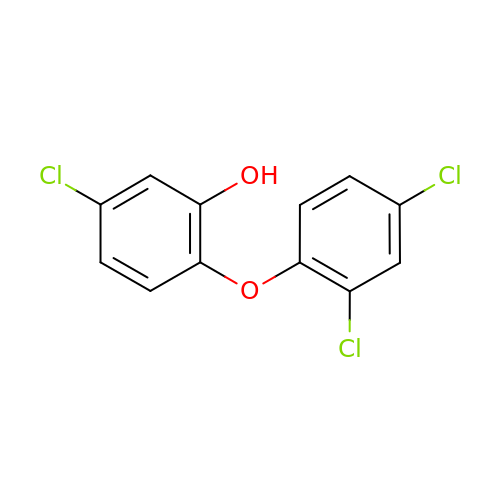TRICLOSAN | C12 H7 Cl3 O2 | XEFQLINVKFYRCS-UHFFFAOYSA-N> MMQGQPHQDAGMPEPYAATADVYDRLVDYAIAEWGECPRPQMADFVEQAWAARGHRVRRVLELCCGTGLMTEQLVRRGYEVTAVDRSETMLALAKQRVGGAADFHQIELPAP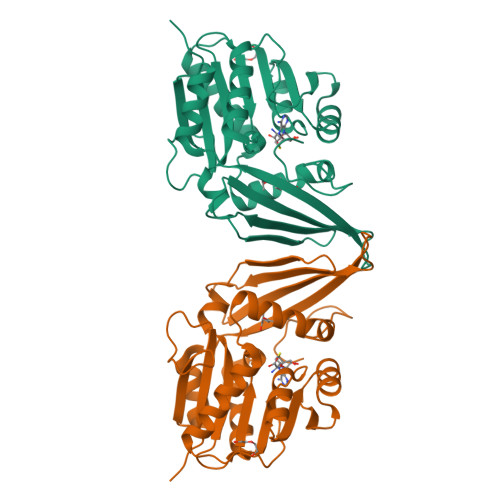LPDGADAVVCTAAAFNYQASARSLGETLRAVATVLPAGATFVFDIETAALLKGHWGNRVWAADEGDLAFIWDFTSEPDTTYCDVHYTQFTRHEAGADAYTGVREVHRLYAFDHDTVRAQARAAGFAQAEVFDNYTERPATDTTRYETWVLTRDERSRHHHHHH> ASSTNLKDVLASLIPKEQARIKTFRQ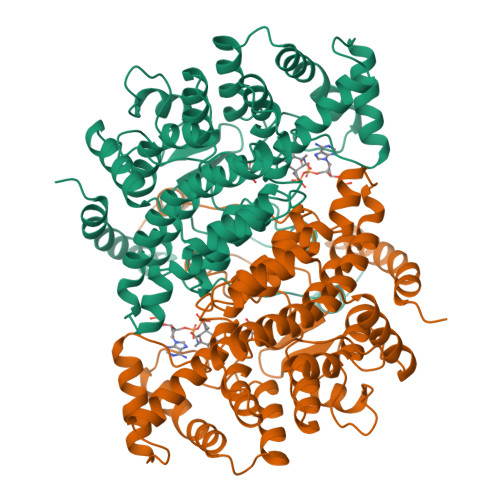QHGNTAVGQITVDMSYGGMRGMKGLIYETSVLDPDEGIRFRGFSIPECQKLLPKAGGGEEPLPEGLFWLLVTGQIPTPEQVSWVSKEWAKRAALPSHVVTMLDNFPTNLHPMSQLSAAITALNSESNFARAYAEGINRTKYWEFVYEDAMDLIAKLPCVAAKIYRNLYRAGSSIGAIDSKLDWSHNFTNMLGYTDPQFTELMRLYLTIHSDHEGGNVSAHTSHLVGSALSDPYLSFAAAMNGLAGPLHGLANQEVLLWLSQLQKDLGADASDEKLRDYIWNTLNSGRVVPGYGHAVLRKTDPRYTCQREFALKHLPSDPMFKLVAQLYKIVPNVLLEQGKAKNPWPNVDAHSGVLLQYYGMTEMNYYTVLFGVSRALGVLAQLIWSRALGFPLERPKSMSTAGLEKLSAGG> MTNRTPRISAIRSAALAALLAGLGMGAAQATEFRSADTHNADDYPTVAAVKYMGELLEKKSGGKHKIKVFNKQALGSEKETIDQVKIGALDFTRVNVGPMNAICPLTQVPTMPFLFSSIAHMRKSLDGPVGDEILKSCESAGFIGLAFYDSGARSIYAKKPIRTVADAKGLKIRVQQSDLWV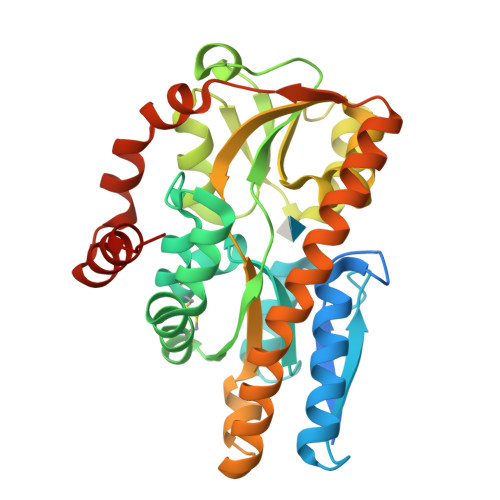ALVSAMGANATPMPYGEVYTGLKTGLIDAAENNIPSFDTAKHVEAVKVYSKTEHSMAPEILVMSKIIYDKLPKAEQDMIRAAAKESVAFERQKWDEQEAKSLANVKAAGAEIVEVDKKSFQAVMGPVYDKFMTTPDMKRLVKAVQDTKAENLYFQ>[4x]SMAPTLSEQTRQLVRASVPALQKHSVAISATMYRLLFERYPETRSLFELPERVIHKLASALLAYARSIDNPSALQAAIRRMVLSHARAGVQAVHYPLVWECLRDAIKEVLGP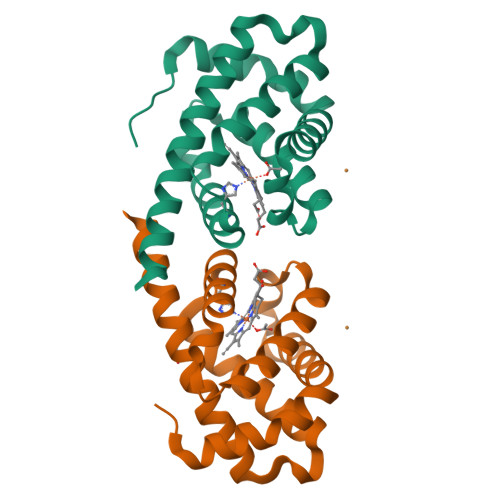DATETLLQAWKEAYDFLAHLLSTKEAQVYAVLAE> QDTSPDTLVVTANRFEQPRSTVLAPTTVVTRQDIDRWQSTSVNDVLRRLPGVDITQNGGSGQLSSIFIRGTNASHVLVLIDGVRLNLAGVSGSADLSQFPIALVQRVEYIRGPRSAVYGSDAIGGVVNIITTRDEPGTEISAGWGSNSYQNYDVSCQQQLGDKTRVTLLGDYAHTHGYDVVAYGNTGTQAQTDNDGFLSKTLYGAL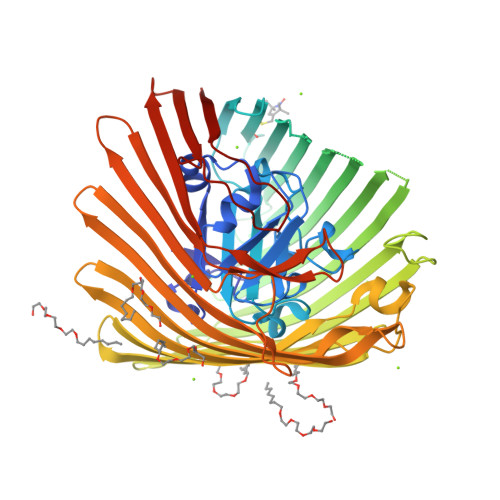EHNFTDAWSGFVRGYGYDNRTNYDAYYSPGSPLLDTRKLYSQSWDAGLRYNGELIKSQLITSYSHSKDYNYDPHYGRYDSSATLDEMKQYTVQWANNVIVGHGSIGAGVDWQKQTTTPGTGYVEDGYDQRNTGIYLTGLQQVGDFTFEGAARSDDNSQFGRHGTWQTSAGWEFIEGYRFIASYGTSYKAPNLGQLYGFYGNPNLDPEKSKQWEGAFEGLTAGVNWRISGYRNDVSDLIDYDDHTLKYYNEGKARIKGVEATANFDTGPLTHTVSYDYVDARNAITDTPLLRRAKQQVKYQLDWQLYDFDWGITYQYLGTRYDKDYSSYPYQTVKMGGVSLWDLAVAYPVTSHLTVRGKIANLFDKDYETVYGYQTAGREYTLSGSYTF(2S)-amino(hydroxy)ethanoic acid | C2 H5 N O3 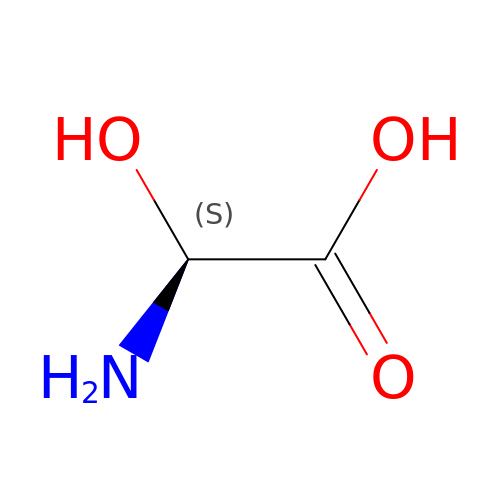| ZHWLPDIRXJCEJY-SFOWXEAESA-N> MRGSHHHHHHGSTANPSLVLNKIDDISFETYDAPEISEPTDVLVQVKKTGICGSDIHFYAHGRIGNFVLTKPMVLGHESAGTVVQVGKGVTSLKVGDNVAIEPGIPCRFCDECKSGHYNLCPHMAFAATPNSKEGEPNPPGTLCKYFKSPEDFLVKLPDHVSLELGALVEPLSVGVHASKLGSVAFGDYVAVFGAGPVGL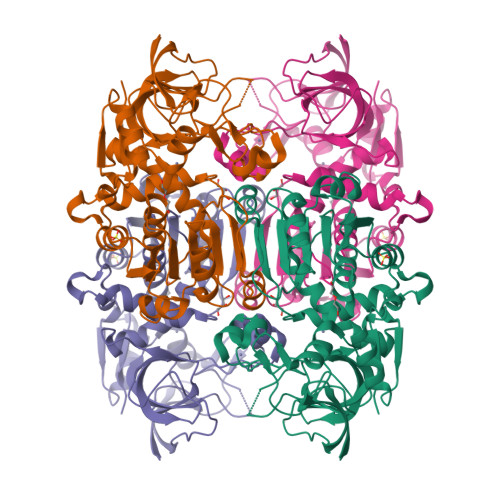LAAAVAKTFGAKGVIVVDIFDNKLKMAKDIGAATHTFNSKTGGSEELIKAFGGNVPNVVLECTGAEPCIKLGVDAIAPGGRFVQVGNAAGPVSFPITVFAMKELTLFGSFRYGFNDYKTAVGIFDTNYQNGRENAPIDFEQLITHRYKFKDAIEAYDLVRAGKGAVKCLIDGPE>[7x]MNLIPTVIEQTNRGERAYDIYSRLLKDRIIMLGSAIDDNVANSIVSQLLFLAAEDPEKEISLYINSPGGSITAGMAIYDTMQFIKPKVSTICIGMAASMGAFLLAAGEKGKRYA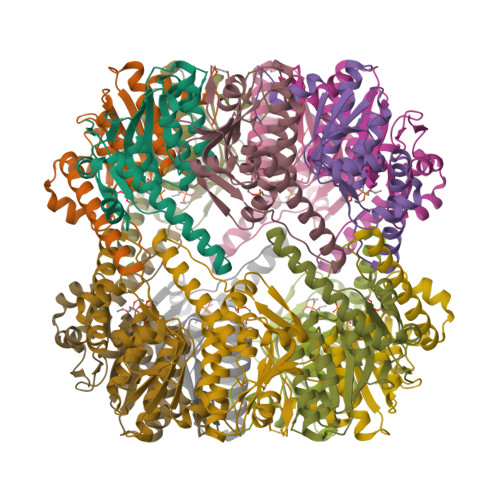LPNSEVMIHQPLGGAQGQATEIEIAAKRILLLRDKLNKVLAERTGQPLEVIERDTDRDNFKSAEEALEYGLIDKILTHTEDKK>QDDASDRQTREVLDPIVASLMEAQQIPGMAIALVRPEGTTISHYGAADRETGTPVDDDTLFEIGSLSKTLTATLASLAEVEGKLDFDAPVSRYLPELEGSAFDDISGLNLGTHTGGGLPLFVPDEVTDRASLMAWYREWQPTEPIGESRTYSNLGIGLLGLETAASLDGEFVPTMRAKVLAPLGMQDTWYDVPEARMADYAMGEDKDGQPTRVSPGVLDDEAYGIKTTAADLAKLVRANLHLADVDAELQQAIDATRQGHYRVGDMTQALIWEQYSLPVAPETLRAGQGYDMILEPNAAEALEPPQSPRDDVWVNKTGSTQGFGGYIVMLPGKHTGLVMLANKNYPNDARVEAAYRILSGLGAIDVP[3x]

To evaluate metal-ion affinity and to identify protein metal-binding sites for Sr2+ and Cs+, a class C β-lactamase (BLA) derived from the moderate halophile Chromohalobacter sp. 560 (HaBLA; molecular weight 39 536) was chosen as a model system. HaBLA, although a moderately halophilic periplasmic protein, has a particularly abundant content of acidic amino acids similar to those in extremely halophilic proteins. The crystal structure of a halophilic β-lactamase from Chromohalobacter sp. 560 (HaBLA) was determined to resolutions of between 1.8 and 2.9 Å in space group P31 using X-ray crystallography. Seven binding sites (site 1 to site 7) for divalent metal ions (Ca2+ and/or Sr2+) and one binding site (site 8) for Cs+ per HaBLA molecule were identified by X-ray diffraction studies including anomalous dispersion.

The NQ-HaBLA crystals soaked into solutions containing Na+, Cs+ and Ca2+ [conditions 1A (0 mM Na+/100 mM Cs+), 1B (75 mM Na+/25 mM Cs+) and 1C (90 mM Na+/10 mM Cs+)] diffracted to resolutions of 2.0, 1.8 and 2.1 Å, respectively. Structural analysis of NQ-HaBLA in condition 1A (0 mM Na+/100 mM Cs+) showed ten locations for bound Ca2+ (Ca1–Ca10) and two locations for Cs+ (Cs1 and Cs2) in an asymmetric unit. The peak heights of the anomalous difference Fourier maps were 17.5σ for Cs1 and 8.0σ for Cs2. The binding sites of Ca2+ were integrated into five sites in one molecule of NQ-HaBLA, which were the same locations as the site 2, site 3, site 5, site 6 and site 7 Ca2+-binding sites in NQ-HaBLA without soaking. Moreover, the binding sites of Cs+ ions were integrated into one site (site 8) per molecule of NQ-HaBLA. The Cs+ ion bound at site 8 was predominantly recognized by two main-chain O atoms and the aromatic ring of Trp189. The aromatic ring of Trp189 interacts with Cs+ by a cation–π interaction. The site 8 Cs+-binding site is not located at the interface of HaBLA molecules but is constructed on the surface of a single HaBLA molecule, indicating that monodisperse HaBLA itself can recognize Cs+.>MAIITPALISALKTSFQKHFQDALATAPSTY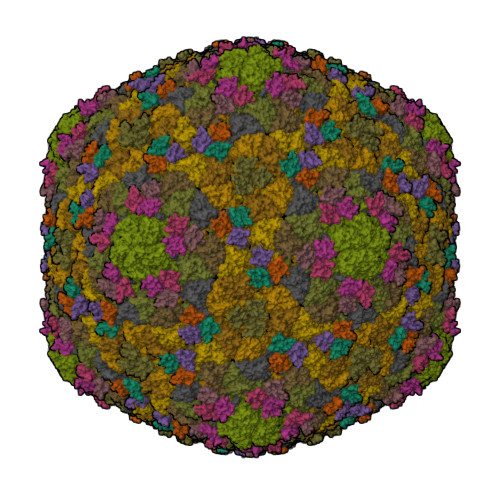LQVATVIPSTTASNTYGWLGQFPKLREWIGQRVIKDMAAQGYQITNKLFESTVGVKRTDIEDDNLGVYGPLMQEMGRAAGAHPDELVFALLKAGNANLCYDGQNFFDTDHPVYPNVDGTGTATTVSNLFAPAADPGAAWYLLDTSRSLKPLIYQERMKPSFTSMTKEDDEQVFMADEYRYGVRSRCNVGFGFWQLAAMSTEELNQVNFEKVYDAMRNQKADGGRPLDIRPNLLVVPTTLRSKAKEVVGVQRLANGADNPNFELVQVLDTAWLN[7x];>[7x]MARQNSAAKTTAKSKTDPATEKPKDDTLPDSTDDASPTAPETPATKPDSASDEVEGVFVRATVERRCRAGFCFDKEGQGFADGVLSDEQLEALESDPLLKVERCTFSGNQEGE Nowadays, the E3 ligase substrate receptor cereblon (CRBN), thalidomide’s primary target, is of particular importance in the fields of MGs and PROTACs. However, these CRBN ligands induce the degradation of IMiD neosubstrates and are inherently unstable, degrading hydrolytically under moderate conditions. In this work, we simultaneously optimized physiochemical properties, stability, on-target affinity, and off-target neosubstrate modulation features to develop novel nonphthalimide CRBN binders. These efforts led to the discovery of conformationally locked benzamide-type derivatives that replicate the interactions of the natural CRBN degron, exhibit enhanced chemical stability, and display a favorable selectivity profile in terms of neosubstrate recruitment.

In 11f, the ortho-fluorine may constitute the major design element, but additional decorations at the benzamide scaffold could prove beneficial. Fortunately, we could study all compounds generated in this iterative step through cocrystal structures in complex with the hTBD homolog MsCI4.44 These data confirmed that the preferred orientation of the ortho substituent toward the amide NH was preserved in the bound state of all ligands except for 11b. Sub van der Waals distances ranging from 1.3 to 2.0 Å were seen in 8d, 11a, 11c, 11d, 11e, and 11f. We determined that F and the NH proton are closely spaced by observing correlation peaks between the NH proton and the F signals in the 19F,1H-HOESY NMR spectra of 8d and 11f. The results, therefore, strongly suggest that IMHBs predetermine the ligand conformation in solution. In addition to the prominent scaffold derived from 8d, we investigated two other hits, 11d and 11f.

>[2x]ASIFRCRQCGQTISRRDWLLPMGGDHEHVVFNPAGMIFRVWCFSLAQGLRLIGAPSGEFSWFKGYDWTIALCGQCGSHLGWHYEGGSQPQTFFGLIKDRLAEGPA;> GASIFRCRQCGQTISRRDWLLPMGGDHEHVVFNPAGMIFRVWCFSLAQGLRLIGAPSGEFSWFKGYDWTIALCGQCGSHLGWHYEGGSQPQTFFGLIKDRLAEGPA>MAASITAITVENLEYPAVVTSPVTGKSYFLGGAGERGLTIEGNFIKFAAIGVYLEDIAVASLAAKWKGKSSEELLETLDFYRDIISGPFEKLIRGSKIRELSGPEYSRKVMENCVAHLKSVGTYGDAEAEAMQKFAEAFKPVNFPPGASVFY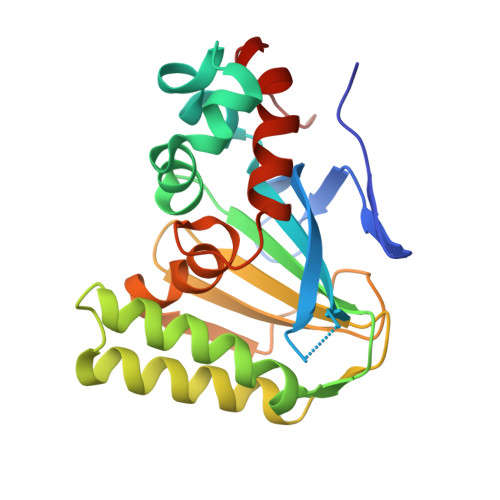RQSPDGILGLSFSPDTSIPEKEAALIENKAVSSAVLETMIGEHAVSPDLKRCLAARLPALLNEGAFKIGN[6x]>[2x]MPFTLGQRWISDTESELGLGTVVAVDARTVTLLFPSTGENRLYARSDSPVTRVMFNPGDTITSHDGWQMQVEEVKEENGLLTYIGTRLDTEESGVALREVFLDSKLVFSKPQDRLFAGQIDRMDRFALRYRARKYSSEQFRMPYSGLRGQRTSLIPHQLNIAHDVGRRHAPRVLLADEVGLGKTIEAGMILHQQLLSGAAERVLIIVPETLQHQWLVEMLRRFNLRF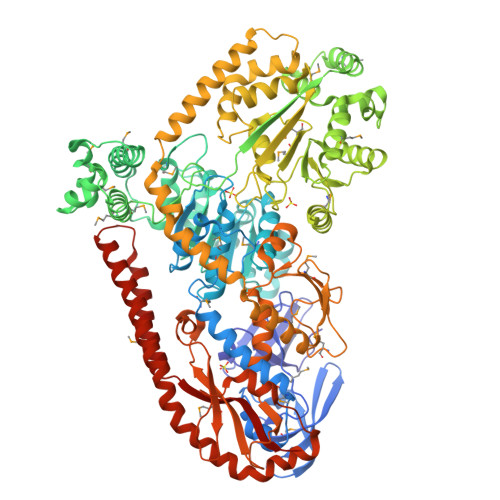ALFDDERYAEAQHDAYNPFDTEQLVICSLDFARRSKQRLEHLCEAEWDLLVVDEAHHLVWSEDAPSREYQAIEQLAEHVPGVLLLTATPEQLGMESHFARLRLLDPNRFHDFAQFVEEQKNYRPVADAVAMLLAGNKLSNDELNMLGEMIGEQDIEPLLQAANSDSEDAQSARQELVSMLMDRHGTSRVLFRNTRNGVKGFPKRELHTIKLPLPTQYQTAIKVSGIMGARKSAEDRARDMLYPERIYQEFEGDNATWWNFDPRVEWLMGYLTSHRSQKVLVICAKAATALQLEQVLREREGIRAAVFHEGMSIIERDRAAAWFAEEDTGAQVLLCSEIGSEGRNFQFASHMVMFDLPFNPDLLEQRIGRLDRIGQAHDIQIHVPYLEKTAQSVLVRWYHEGLDAFEHTCPTGRTIYDSVYNDLINYLASPDQTEGFDDLIKNCREQHEALKAQLEQGRDRLLEIHSNGGEKAQALAESIEEQDDDTNLIAFAMNLFDIIGINQDDRGDNMIVLTPSDHMLVPDFPGLSEDGITITFDREVALAREDAQFITWEHPLIRNGLDLILSGDTGSSTISLLKNKALPVGTLLVELIYVVEAQAPKQLQLNRFLPPTPVRMLLDKNGNNLAAQVEFETFNRQLNAVNRHTGSKLVNAVQQDVHAILQLGEAQIEKSARALIDAARNEADEKLSAELSRLEALRAVNPNIRDDELTAIESNRQQVMESLDQAGWRLDALRLIVVTHQ>[4x]MGHHHHHHMESVTVYAAASLTNAINDLEKIYEKQNKVEVKTSYAGSSTLAKQIEAGAPADIFISADTQWMDYLQNKKLVAANDRINLLGNRLVLITPKGQSLNIKLDKAT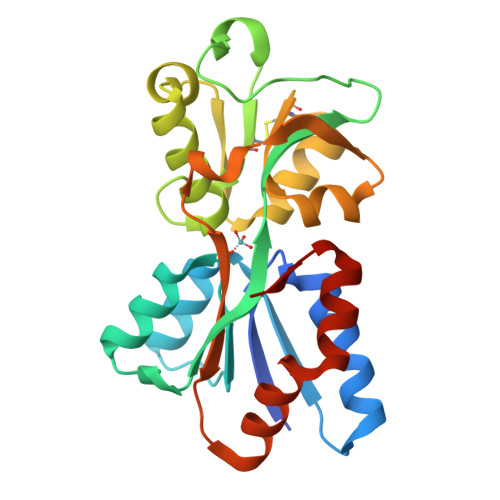DPNKVFTGKICTGDTKSVPVGKYAKQAFTNLGWWNRIEPKLVETEDVRVALNFVARGECQVGIVYATDAAISKDVKVAGIFPENTHSPIIYPLGLIKKNSNSAKFYQFLQSNQAKAVFKKYGFSMLAPVKP A stilbene O-methyltransferase, SbSOMT, is first shown to be indispensable for pathogen-inducible pterostilbene (3,5-bis-O-methylated) biosynthesis in sorghum (Sorghum bicolor). Phylogenetic analysis indicates the recruitment of genus-specific SOMTs from canonical caffeic acid O-methyltransferases (COMTs) after the divergence of Sorghum spp. from Saccharum spp. In recombinant enzyme assays, SbSOMT and COMTs regioselectively catalyze O-methylation of stilbene A-ring and B-ring respectively. Whilst SbSOMT shows global structural resemblance to SbCOMT, molecular characterizations illustrate two hydrophobic residues (Ile144/Phe337) crucial for substrate binding orientation leading to 3,5-bis-O-methylations in the A-ring. The catalytic residues of SbSOMT are highly conserved with all reported COMTs, including His282 as the key nucleophile, whereas Asp283, Glu310, and Glu342 collectively charge the basicity or confine His282 in its reactive conformation.

To rationalize their different catalytic regioselectivities, structural analyses involving X-ray crystallography and computational methods were conducted. We solved the crystal structure of an SbSOMT-resveratrol-nicotinamide adenine dinucleotide (β-NAD) ternary complex (diffracted to 1.72 Å resolution, Fig. 4d; β-NAD was utilized as an additive to improve crystallization), an SbSOMT-resveratrol binary complex, and two ternary complexes reproduced with pinostilbene or pterostilbene (diffracted at 2.10 and 2.56 Å, respectively). All complexes were in high structural resemblance and depicted as a homodimer with an open conformation. Superimposition of SbSOMT and SbCOMT (PDB: 4PGH21) revealed their high structural similarity (RMSD = 2.322 Å), except that SbSOMT harbors an extended loop (Val103-Cys114) that forms a threonine-rich dimerization interface. Close examination of the SbSOMT substrate binding pocket within the SbSOMT-resveratrol-β-NAD complex provided further insights into the interactions between SbSOMT and its stilbene substrates. The pocket mainly comprised hydrophobic residues, and the stilbene backbone was secured by hydrophobic interactions with Met143, Ile144, Met175, Phe189, Met193, Trp279, Tyr311, Leu329, Met333, Thr336, in addition to Leu28 of the adjacent protomer. The apparent binding cavity was confined to fit the stilbene backbone in a planar configuration with minimal rotational flexibility. Of the three hydroxyl groups on resveratrol capable of forming hydrogen bonds, only the methyl-accepting 3-OH group (A-ring) formed direct hydrogen bonds to SbSOMT residues, including the catalytic residues His282 (2.80 Å) and Asp283 (3.26 Å). Other hydroxyl groups were shielded by water molecules and did not directly interact with SbSOMT. Overall, these structures depicted a productive substrate orientation within the substrate binding pocket which greatly favors A-ring O-methylation.

>[2x]MGSYDSSSSSSNDSSARNEEDESCMFALKLLGGFAVPFTIKAVIELGVMDQLLTAERAMSAEELVAAAVAAQLPRPEVACTMVDRLLRFLASHSVVRCTTEVVVGTDDATTTTCCRRSYAASPVCKWFARNGVEDSVLPLGMMILNKTFLDSWQNITDAVLEGAAPFEKTYGMPMFEYLSTNGPLNTVFHEAMANHSMIITKKLLKFFRGFEGLDVLVDVGGGNGTTLQMIRGQYKNMRGINYDLPHVIAQAAPVEGVEHVGGSMFDNIPRGNAVLLKWILHDWDDKACIKILKNCYTALHVRGKVIVLEYVVPDEPEPTLAAQGAFELDLTMLVTFGSGKERTQREFSELAMEAGFSREFKATYIFANVWALEFTK> APAVPNKPVEVKGSQKTVMFPHAPHEKVECVTCHHLVDGKESYAKCGSSGCHD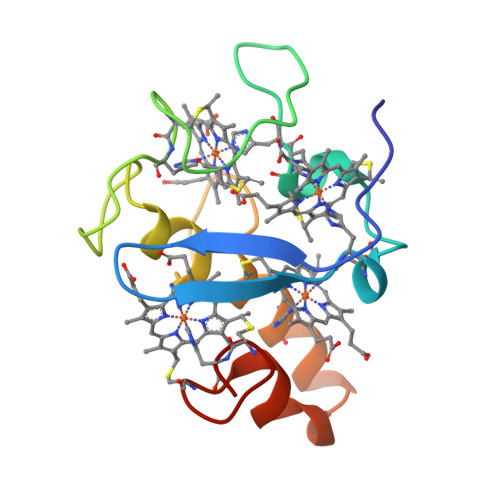DLTAKKGEKSLYYVVHAKGELKHTSCLACHSKVVAEKPELKKDLTGCAKSKCHP>SMDVGVVGLGVMGANLALNIAEKGFKVAVFNRTYSKSEEFMKANASAPFAGNLKAFETMEAFAASLKKPRKALILVQAGAATDSTIEQLKKVFEKGDILVDTGNAHFKDQGRRAQQLEAAGLRFLGMGISGGEEGARKGPAFFPGGTLSVWEEIRPIVEAAAAKADDGRPCVTMNGSGGAGSCVKMYHNSGEYAILQIWGEVFDILRAMGLNNDEVAAVLEDWKSKNFLKSYMLDISIAAARAKDKDGSYLTEHVMDRIGSKGTGLWSAQEALEIGVPAPSLNMAVVSRQFTMYKTERQANASNAPGITQSPGYTLKNKSPSGPEIKQLYDSVCIAIISCYAQMFQ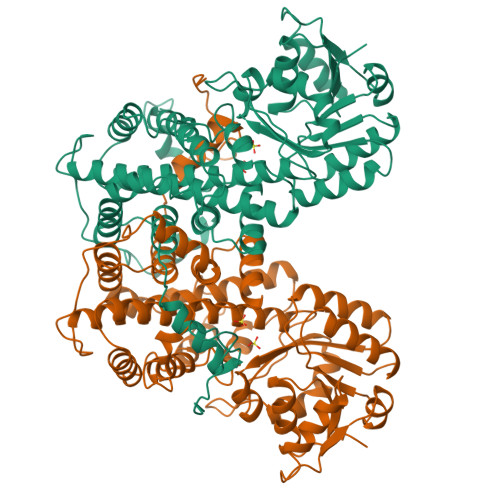CLREMDKVHNFGLNLPATIATFRAGCILQGYLLKPMTEAFEKNPNISNLMCAFQTEIRAGLQNYRDMVALITSKLEVSIPVLSASLNYVTAMFTPTLKYGQLVSLQRDVFGRHGYERVDKDGRESFQWPELQ[2x]> MATRLDRLVTILETGSTRLIRDTAVNQLADWQKQHPEELFNLLSRVVPYLRHKDWETRTTAAKAIGKIIENAPLYDPNAGQDEAAPEP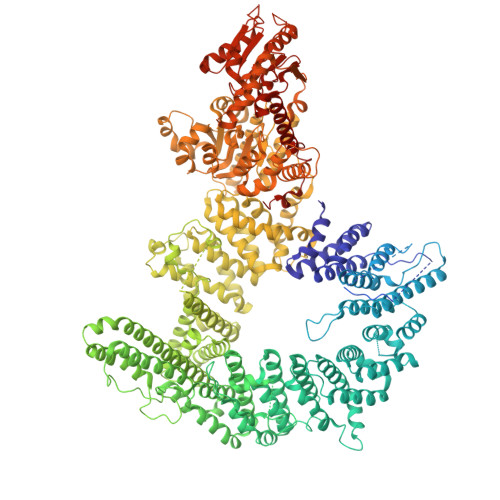TNGSFEVKKEEEKDVLEQDNFFRLESLDVATIVKYGRPLLRGGPVDYNLAALDPQKRLAHLKKTLNGRLGLLGRVFEDEEMPVEQIASPITPNDAAGANGVGRQDGASNDNQSQAIDESKMSARQLNVLKRKRKREAQKAAQGKSGFGDLSLRRSTTAGSDAFGEDTPMPDADSKKNKLAEYFSLDRPENTEEDTKIVSEFKGPVLPIKSEIEADDSLEGAEWPFERLCEFLKVDLFDPQWETRHGAAMGLREVIRVHGAGAGRRRGKTRKENNDLNRQWLDDLAYRLLCVLMLDKFTDYSSDTSVAPIRETVGQTLGAVLRHISVESVHAIYRLLYCMVTQEDLPSEQNMWAVCHGGMVGLRYVVAVRKDLLLQDGDMIDGVVRCVMQGLGDIDDDVRSVSAATLIPMAKEFVMMRRSALDSLINIVWESLSNLGDDLSASTGKIMDLLATLCSFPEVLEAMKVSASQDEERSFTLLVPRLYPFLRHTITSVRLAVLKALMTFANLGGETSQGWLNGRILRLIFQNIIVERDQDTLNMSLELWTTLVRRLAARDPAILADEFEAHAEPMMQLALHPIGVPRHPIPMNPALFQKPSGGTYSLPGASQTNSRRSSPPEGERATKRRRKSTKAEDVAPSTHTHDVDGHMIQGEVDLVGVDVLIRSRISAAKAMGLIMSFIPTPRLASYDTAVLQALSSPYASTQLAAAMVIDEYAKNCSTPEVASRFIEPLQKIIDLERPSHYRDLVTYVQRVRSASQQLINLFRDHGKVSQGKLPTLAVVVQGEPEAGPGAFSIANAEKVVNEDFERLKRLMAPGQRLIALPQLNEAREQTVEVIEEAKAAKEARDARIKAAAACALVAMKVLPKKPSPLIKAIMDSIKTEENQELQSRSAATIARLVQLFTESGRRGPAEKVVANLVKFSCVEVAETPEFPIHAHKTNVILSMQKEEDRVDHPDAVKYAREAKAARITRRGAKEALEILSKNFGAELLERVPTLRTFMEEPLVRAFSGDLPPEARDPENAFGQEIVDAMSVIRTMTPTLHPALHPFVMQQVPLVIKALRSDLSVFRYMAAKCMATICSVITVDGMTALVEKVLPSINNPLDLSFRQGAIEVIYHLIAVMGDAILPYVIFLIVPVLGRMSDSDNQIRLIATTSFATLVKLVPLEAGIPDPPGLSEELLKGRDRERTFIAQLLDPKKIEPFKIPVAIKAELRSYQQEGVNWLAFLNKYHLHGILCDDMGLGKTLQTICIVASDHHQRAEEFARTGAPEVRKLPSLIICPPTLSGHWQQEIKTYAPFLTVTAYVGSPAERRAMKDSLDKTDIVITSYDVCRNDIDVIEKYNWNYCVLDEGHLIKNPKAKITLAVKRLTSNHRLILTGTPIQNNVLELWSLFDFLMPGFLGAEKVFLDRFAKPIANSRYSKASSKEQEAGALAIEALHKQVLPFLLRRLKEEVLNDLPPKILQNYYCDLSDLQRKLFEDFTKREGKKITETAGRDDKEAKQHIFQALQYMRKLCNSPALVMKPGHKAYEDTQKYLAKHGTTLEDPIHAPKLGALRDLLVDCGIGVEGQESSDPLYTPIKPHRALIFCQMKEMLDMVQNTVLKQMLPSVSYLRLDGSVEANKRQDIVNKFNSDPSYDVLLLTTSVGGLGLNLTGADTVIFVEHDWNPQKDLQAMDRAHRIGQKKVVNVYRIITRGTLEEKILSLQRFKIDVASTVVNQQNAGLATMDTDQILDLFNLGESGPSLITDNKESIEAAAWSHPQFEK> MKDLVDTTEMYLRTIYELEEEGVTPLRARIAERLEQSGPTVSQTVARMERDGLVVVASDRSLQMTPTGRTLATAVMRKHALAERLLTDIIGLDINKVHDEACRWEHVMSDEVERRLVKVLKDVSRSPFGNPIPGLDELGVGNSDAAAPGTRVIDAATSMPRKVRIVQINEIFQVETDQFTQLLDADIRVGSEVEIVDR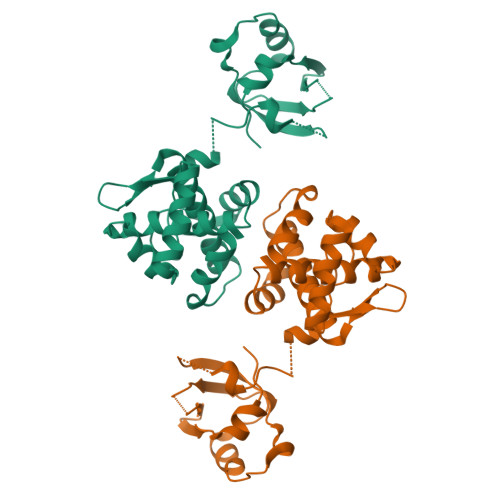DGHITLSHNGKDVELLDDLAHTIRIEEL>MWVKILSVVGARPQFIKAAAVSRVLRASPGVREVLVHTGQHYDDNMSQVFFEELEIPDPDYHLGIGGGTHGQNTGRMLEAIEGVLLKEKPDWVLVYGNTDSTLAGALAAVKLHIPVAHVEAGLRSFNRRMPEEINRILTDHASDLLFAPTETAVQNLLREGIPENRIHLVGDVMYDAALHYGAKAERKSRILERLGLQAKGYVLATIHRAENTDDQERLRVILEALAEVHQEVPVVFPVHPRTRKRAEAFGLGSYLEKVVALEPVGYLDMVMLEKNARLIVTDSGGVQKEAYFYRVPCVTVREETEWVELLKAEWNYLAAPQNAKDLALTILHRMRTKGVEIDLYGDGRASQKISDFLRKVGIRTLEHHHHH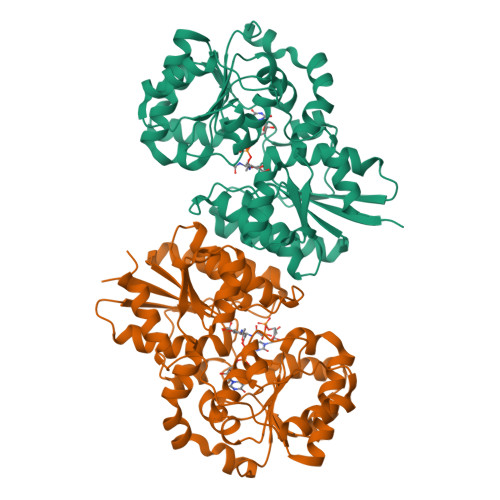H[2x]> MAMSNMTYNNVFDHAYEMLKENIRYDDIRDTDDLHDAIHMAADNAVPHYYADIFSVMASEGIDLEFEDSGLMPDTKDVIRILQARIYEQLTID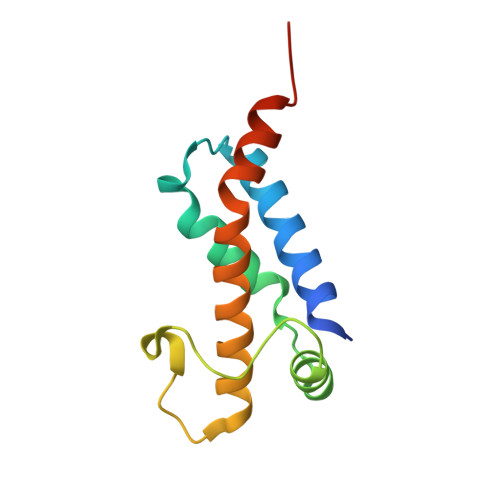LWEDAEDLLNEYLEEVEEYEEDE2-(difluoromethyl)-1H-benzimidazole | C8 H6 F2 N2 | 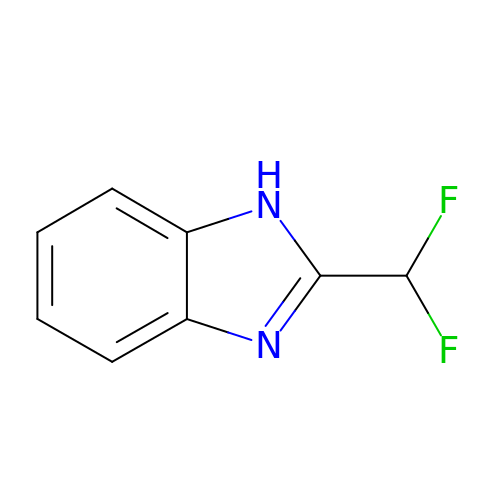PURNIHSRWGYONZ-UHFFFAOYSA-N>MELIRIAMKKDLENDNSLMNKWATVAGLKNPNPLYDFLNHDGKTFNEFSSIVNIVKSQYPDREYELMKDYCLNLDVKTKAARSALEYADANMFFEIEDVLIDSMISCSNMKSKEYGKVYKIHRELSNSVITEFEAVKRLGKLNIKTPEMNSFSRLLLLYHYLSTGNFSPMAQLIKQIDLSEI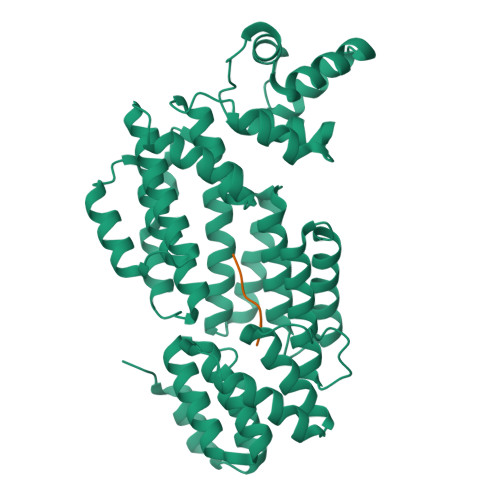SENMYIRNTYQTRVHVLMSNIKLNENSLEECREYSKKALESTNILRFQVFSYLTIGNSLLFSNYELAQENFLKGLSISVQNENYNMIFQQALCFLNNVWRKENKWINFESDSIMDLQEQAHCFINFNENSKAKEVLDKLDLLVHNDNELAMHYYLKGRLEQNKACFYSSIEYFKKSNDKFLIRLPLLELQKMGENQKLLELLLLLEYA[2x];>GMPRGA[2x]> GSGAMAATYSALNSSK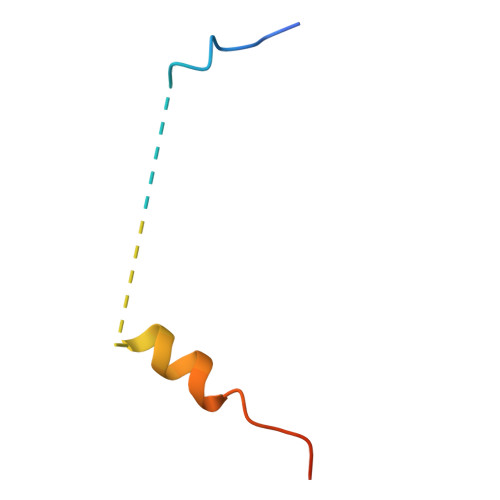PTPQLKPIESSILAQRRVRKLPSTTL Microbes use a diverse set of metal-specific sensors known as metalloregulatory proteins to respond to changes in metal concentration in the immediate environment. Zinc uptake regulator (Zur) is a homolog of one of the first metalloregulatory proteins identified, namely the ferric uptake regulator protein (Fur). Each EcZur monomer includes two domains: an N-terminal DNA-binding domain and a C-terminal dimerization domain. The DNA-binding domain (α2–α4) contains a helix-turn-helix (HTH) motif and is connected to the C-terminal domain (α5/β5) using a characteristic winged-helix motif.

The structure of E. coli Zur (EcZur) protein in complex with a 31 bp duplex derived from the znuABC operator (PznuABC) was determined by X-ray crystallography using multiwavelength anomalous dispersion (MAD) data collected at both high energy and the zinc absorption edge and refined to 2.50 Å. Analysis of the complex reveals the HTH motif interacts with the major and minor grooves of the DNA. Figure 1 shows the final model which includes amino acid residues 5–152 of four protein monomer chains (designated chains A, B, C, D), eight zinc ions, and two 31 bp strands of DNA (designated chains Y and Z) in the asymmetric unit. The three dimensional model of the complex shows the central portion of the operator DNA surrounded by four Zur monomers forming a dimer of dimers. The nature of the dimer of dimers ((Zur2)2) structure indicated that there were two possible orientations for the DNA to adopt in the crystal. Using DNA brominated at asymmetric points indicated that the crystal has an equal mixture of both DNA orientations. Given the pseudo-palindromic nature of the DNA sequence none of the protein-DNA contact sites were affected by this lack of directionality; however, several bases represent an average over the two conformations. Anomalous difference data collected at the Zn edge reveal two distinct Zn2+ binding sites in each of the four Zur monomers: the Zn2+ in site A is bound to four sulfur atoms from Cys103, Cys106, Cys143, and Cys146 and the Zn2+ in site B is bound by residues His77, Cys88, His96, and Glu111. Each monomer A through D has two hydrogen bond donors, Tyr45 and Arg65, that interact with the N7 nitrogen of bases G7, A11′, A12, A15, A16′, G19′, A20, G24′ (where ′ denotes non-coding strand). Each of the four monomers recognizes two purines on opposite strands of DNA separated by three base pairs in an R-N-N-N-Y motif. Two salt bridges between adjacent dimers were observed, between Asp49 from monomer A to Arg52 of monomer B, and vice versa.

>[4x]MEKTTTQELLAQAEKICAQRNVRLTPQRLEVLRLMSLQDGAISAYDLLDLLREAEPQAKPPTVYRALDFLLEQGFVHKVESTNSYVLCHLFDQPTHTSAMFICDRCGAVKEECAEGVEDIMHTLAAKMGFALRHNVIEAHGLCAACVEVEACRHPEQCQHDHSVQVKKKPR>[2x]GPMSSVQLSRGDFHSIFTNKQRYDNPTGGVYQVYNTRKSDGANSNRENLIMISDGIYHMKALLRNQAASKFQSMELQRGDIIRVI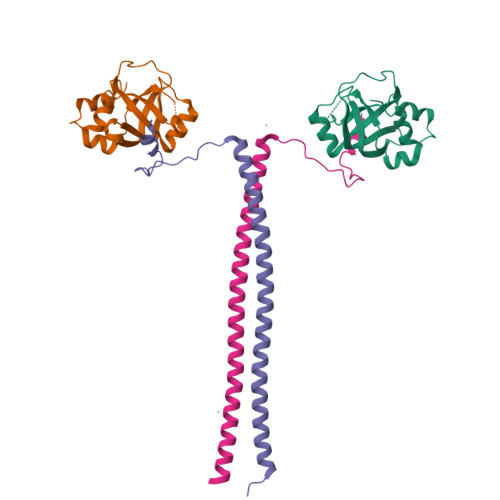IAEPAIVRERKKYVLLVDDFELVQSRADMVNQTSTFLDNYFSEHPNETL;>[2x]GPMADLWDDNDDDDDILELVNRPPMSQMAVPIKPPESQAEQLMKAKGEVGVLRQKLSMLEKTLREHDDNQKKLESSLKSSHEEEVTKLKIELERLEDERKFMLLEQKHLFT>[3x]GSFVEMVDNLRGKS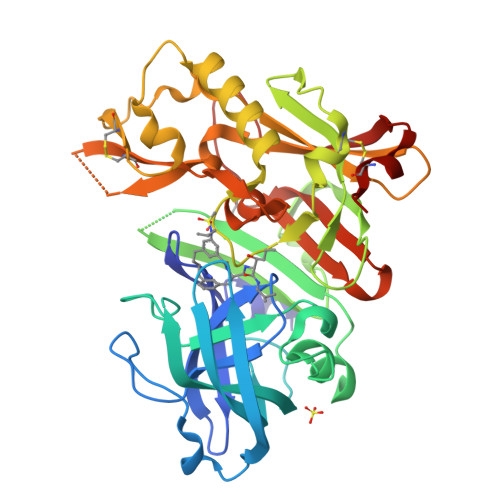GQGYYVEMTVGSPPQTLNILVDTGSSNFAVGAAPHPFLHRYYQRQLSSTYRDLRKGVYVPYTQGKWEGELGTDLVSIPHGPNVTVRANIAAITESDKFFINGSNWEGILGLAYAEIARPDDSLEPFFDSLVKQTHVPNLFSLQLCGAGFPLNQSEVLASVGGSMIIGGIDHSLYTGSLWYTPIRREWYYEVIIVRVEINGQDLKMDCKEYNYDKSIVDSGTTNLRLPKKVFEAAVKSIKAASSTEKFPDGFWLGEQLVCWQAGTTPWNIFPVISLYLMGEVTNQSFRITILPQQYLRPVEDVATSQDDCYKFAISQSSTGTVMGAVIMEGFYVVFDRARKRIGFAVSACHVHDEFRTAAVEGPFVTLDMEDCGYNI> PNFSGNWKIIRSENFEELLKVLGVNVMLRKIAVAAASKPAVEIKQEGDTFYIKTSTTVRTTEINFKVGEEFEEQTVDGRPCKSLVKWESENKMVCEQKLLKGEGPKTSWTRELTN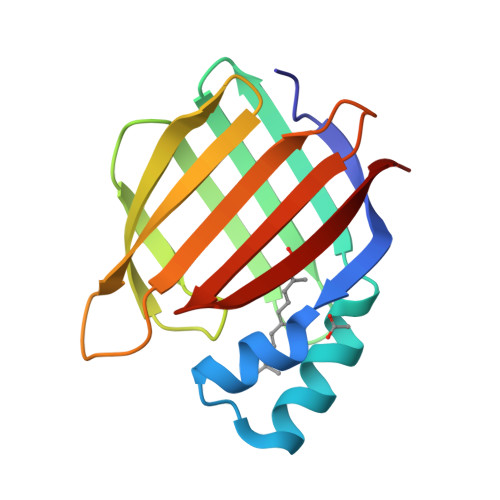DGELILTMTADDVVCTRVYVRE In this work, we exhaustively probe the ability of all 36 immobile HJ sequences to form DNA crystals in two different designed systems. Three separate self-assembling DNA crystal systems are described in this report: the “4 × 5” and “4 × 6” designs (collectively referred to as the 4 × N systems), and a third construct with a “scrambled” sequence variant of the 4 × 6 lattices. Self-assembly was mediated by three constituent oligonucleotides: (S1) containing four sequence repeats of either 5 or 6 bases; (S2) composed of 21 bases containing complementary regions to both (S1); and (S3) which forms the second junction crossover. The HJ serves as the fundamental component at the core of each unit, and the ultimate assembly of the full lattice is facilitated by the complementary 2-base sticky ends that tail each duplex.

To investigate this possibility, we designed “scrambled” sequences with targeted base substitutions, while maintaining GC content, along each “stem”. Contrary to the buffer preference observed with the native P32 crystals, the scrambled systems exhibited an exclusive preference towards low salt buffers, much like the native R3 crystals. Remarkably, only J1 and J2 retained the P32 symmetry, with all others yielding an R3 lattice. There appeared to be only a marginal difference in the average cell lengths in the R3 scramble crystals (a = b = 113.04 c = 51.10) relative to the native 4 × 6 sequences: the a, b axis trended ~2 Å shorter and c ~1.3 Å longer, whereas in the J1 and J2 cases, the crystals were in good agreement with the original 4 × 6 motif. The average angles of the R3 and P32 crystals were 61.00° (σ = 1.21) and 58.05° (σ = 1.39), respectively. However, in the majority of the crystal structures reported here, the cacodylate anion indeed fits best into the electron density map of our X-ray structures, due to the presence of sodium cacodylate in the crystallization solution.

> GAACGACAGAGA;> CGTCGACTC;> TCTACG;> TCGAGTCGCTGTCGT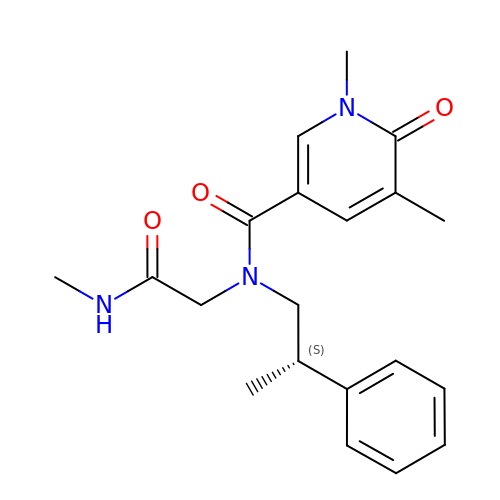1,5-dimethyl-N-[2-(methylamino)-2-oxidanylidene-ethyl]-6-oxidanylidene-N-[(2S)-2-phenylpropyl]pyridine-3-carboxamide | C20 H25 N3 O3 | HZVLFNBTVSYMSI-OAHLLOKOSA-N> TTCCP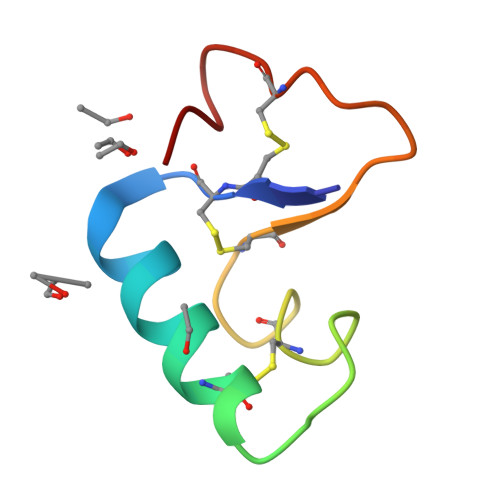SIVARSNFNVCRLPGTPEALCATYTGCIIIPGATCPGDYAN>[3x]GMGKEIEIERKTLVSKETFKRLISQLHIGEGDFKLQRNHYF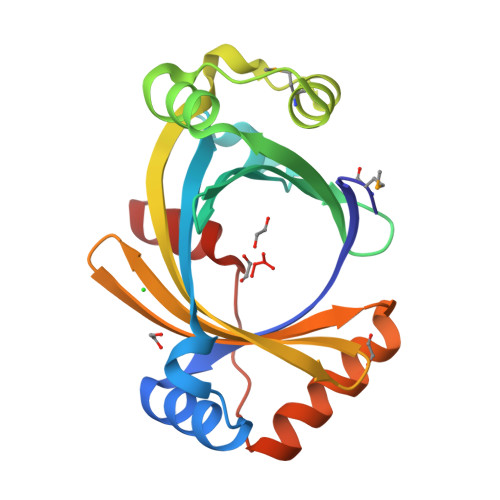ETDDFQLKKQSSALRIREKEAIFTFTLKQPHPAGLLETNQTLSKQEAKLALESAHFPSGEVMDALRDLSIPISQLKHIGTLSTSRAEISYEQGILCLDHSSYLGIEDYEIEFEGTSEEHATVTFQEILKTFSISQVPTENKIQRFFSKKEKN>[4x]GSASPTP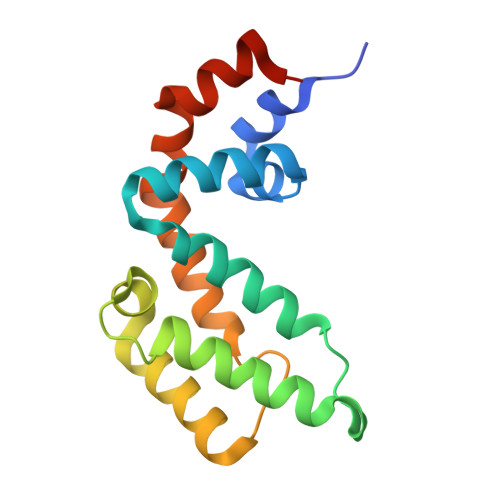PYLKWAESLHSLLDDQDGISLFRTFLKQEGCADLLDFWFACTGFRKLEPCDSNEEKRLKLARAIYRKYILDNNGIVSRQTKPATKSFIKGCIMKQLIDPAMFDQAQTEIQATMEENTYPSFLKSDIYLEYTRTGSESPKV> GSGIIEFHVIGNSLTPKANRRVLLWLVGLQNVFSHQLPRMPKEYIARLVFDPKHKTLALIKDGRVIGGICFRMFPTQGFTEIVFCAVTSNEQVKGYGTHLMNHLKEYHIKHNILYFLTYADEYAIGYFKKQGFSKDIKVP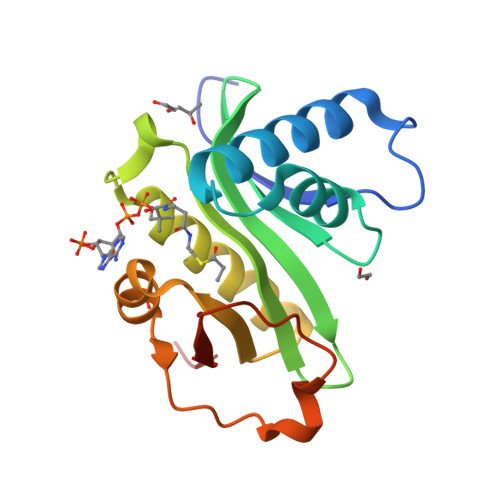KSRYLGYIKDYEGATLMECELNPRIPYT> VTFDVGDEYEIIETIGNGAYGVVSSARRRLTGQQVAIKKIPNAFDVVTNAKRTLRELKILKHFKHDNIIAIKDILRPTVPYGEFKSVYVVLDLMESDLHQIIHSSQPLTLEHVRYFLYQLLRGLKYMHSAQVIHRDLKPSNLLVNENCELKIGDFGMARGLCTSPAEHQYFMTEYVATRWYRAPELMLSLHEYTQAIDLWSVGCIFGEMLARRQLFPGKNYVHQLQLIMMVLGTPSPAVIQAVGAERVRAY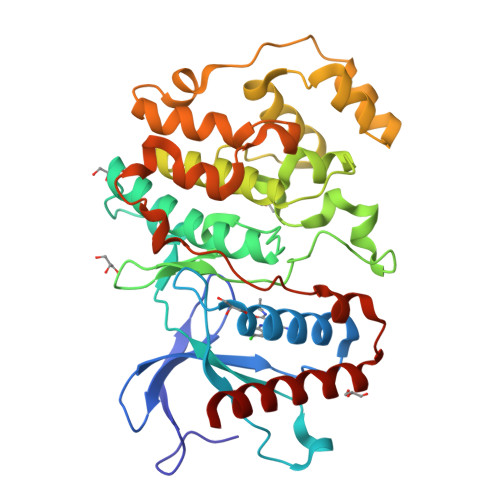IQSLPPRQPVPWETVYPGADRQALSLLGRMLRFEPSARISAAAALRHPFLAKYHDPDDEPDCAPPFDFAFDREALTRERIKEAIVAEIEDFHARRE> MNWLF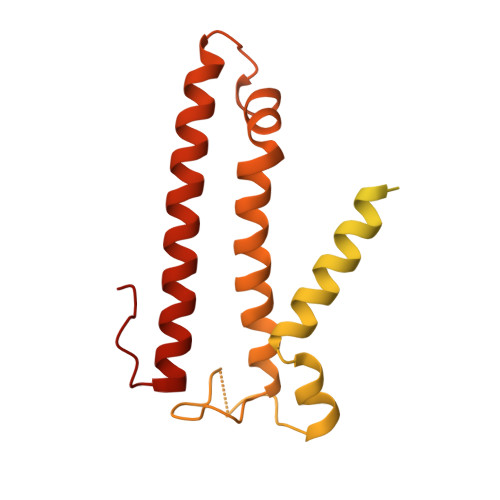LVSLVFFCGVSTHPALAMSSNRLLKLANKSPKKIIPLKDSSFENILAPPHENAYIVALFTATAPEIGCSLCLELESEYDTIVASWFDDHPDAKSSNSDTSIFFTKVNLEDPSKTIPKAFQFFQLNNVPRLFIFKPNSPSILDHSVISISTDTGSERMKQIIQAIKQFSQVNDFSLHLPMDWTPIITSTIITFITVLLFKKQSKLMFSIISSRIIWATLSTFFIICMISAYMFNQIRNTQLAGVGPKGEVMYFLPNEFQHQFAIETQVMVLIYGTLAALVVVLVKGIQFLRSHLYPETKKAYFIDAILASFCALFIYVFFAALTTVFTIKSPAYPFPLLRLSAPFK>[2x]DYDIPTTENLYFQGSMSRPIVISGPSGTG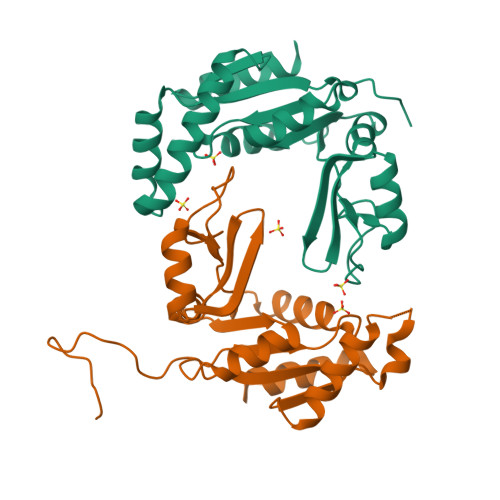KSTLLKKLFAEYPDSFGFSVPSTTRTPRAGEVNGKDYNFVSVDEFKSMIKNNEFIEWAQFSGNYYGSTVASVKQVSKSGKTCILDIDMQGVKSVKAIPELNARFLFIAPPSVEDLKKRLEGRGTETEESINKRLSAAQAELAYAETGAHDKVIVNDDLDKAYKELKDFIFAEK>[2x]GSHMVTIVRIYLDGVYGIGKSTTGRVMASAASGGSPTLYFPEPMAYWRTLFETDVISGIYDTQNRKQQGNLAVDDAALITAHYQSRFTTPYLILHDHTCTLFGGNSLQRGTQPDLTLVFDRHPVASTVCFPAARYLLGDMSMCALMAMVATLPREPQGGNIVVTTLNVEEHIRRLRTRARIGEQIDITLIATLRNVYFMLVNTCHFLRSGRVWRDGWGELPTSCG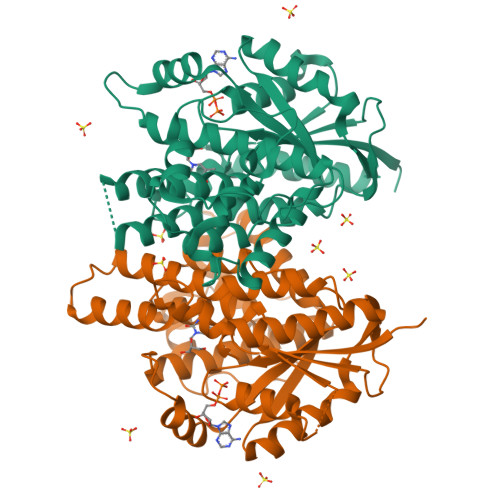AYKHRATQMDAFQERVSPELGDTLFALFKTQELLDDRGVILEVHAWALDALMLKLRNLNVFSADLSGTPRQCAAVVESLLPLMSSTLSDFDSASALERAARTFNAEMGV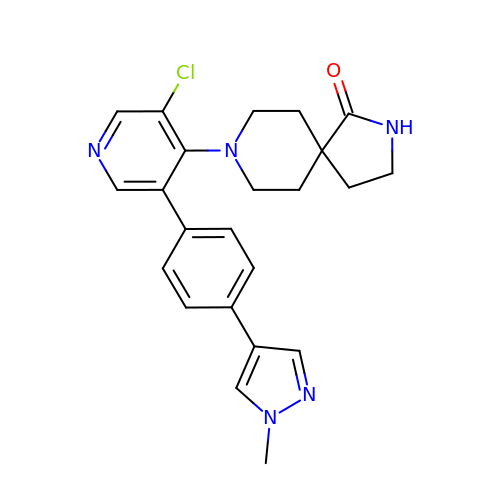8-{3-chloro-5-[4-(1-methyl-1H-pyrazol-4-yl)phenyl]pyridin-4-yl}-2,8-diazaspiro[4.5]decan-1-one | C23 H24 Cl N5 O | LBFYQISQYCGDDW-UHFFFAOYSA-N>[4x]MASRGVNKVILVGNLGQDPE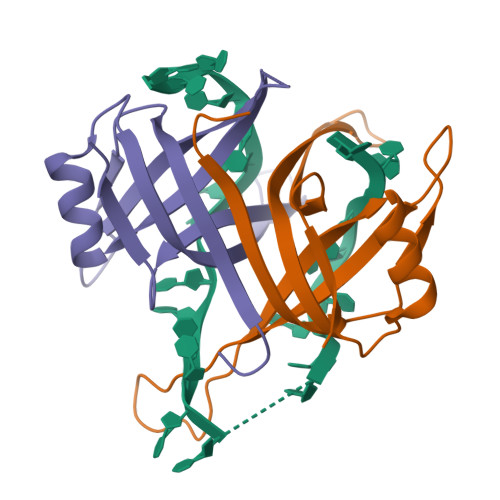VRYMPNGGAVANITLATSESWRDKATGEMKEQTEWHRVVLFGKLAEVASEYLRKGSQVYIEGQLRTRKWTDQSGQDRYTTEVVVNVGGTMQMLGGR> GSFIDIEFPEWFHEGLSRHQAENLLMGKDIGFFIIRASQSSPGDFSISVRHEDDVQHFKVMRDTKGNYFLWTEKFPSLNK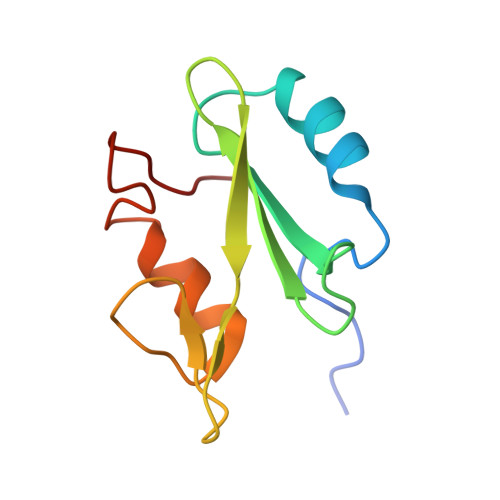LVDYYRTTSISKQKQVFLRD> MRVNNGLTPQELEAYGISDVHDIVYNPSYDLLYQEELDPSLTGYERGVLTNLGAVAVDTGIFTGRSPKDKYIVRDDTTRDTFWWADKGKGKNDNKPLSPETWQHLKGLVTRQLSGKRLFVVDAFCGANPDTRLSVRFITEVAWQAHFVKNMFIRPSDEELAGFKPDFIVMNGAKCTNPQWKEQGLNSENFVAFNLTERMQLIGGTWYGGEMKKGMFSMMNYLLPLKGIASMHCSANVGEAGDVAVFFGLSGSGKTTLSTDPARRLIGDDEHGWDDDGVFNFEGGSYAKTIKLSKEAEPEIYAAIRRDALLENVTVRAGGTIDFDDGSKTENTRVSYPIYHIDNIVKPVSKAGHATKVIFLTADAFGVLPPVSRLTADQTQYHFLSGFTAAAAGTERGITEPTPTFSACFGAAFLSLHPTQYAEVLVKRMQAAGAQAYLVN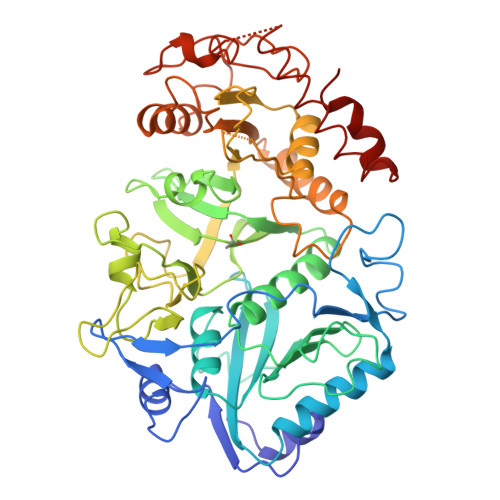TGWNGTGKRISAADTRAIIDAILNGSLDNAETFTLPMFNLAIPTELPGVDTGILDPRNTYASPAGWQEKAETLAKLFIDNFDKYTDTPAGAALVAAGPAL(3~{R},5~{S})-5-[(2~{R})-2-[(1~{R},3~{a}~{S},4~{Z},7~{a}~{R})-7~{a}-methyl-4-[(2~{E})-2-[(3~{S},5~{R})-2-methylidene-3,5-bis(oxidanyl)cyclohexylidene]ethylidene]-2,3,3~{a},5,6,7-hexahydro-1~{H}-inden-1-yl]propyl]-3-methyl-3-oxidanyl-1-(2-phenylethyl)pyrrolidin-2-one | C35 H49 N O4 | 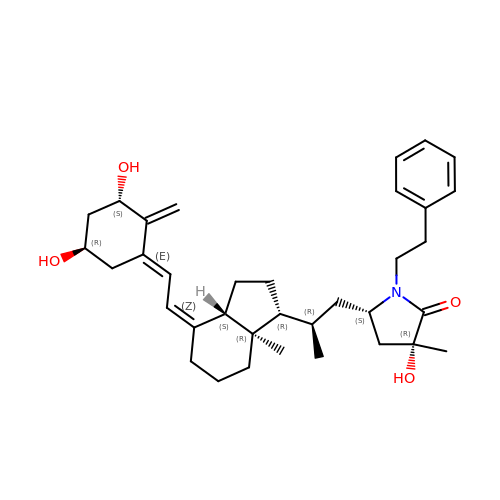KMTLDHCLGFVLKS-YMDIQGDRSA-N>GMATVRLLDDAEISTLPEVKAVFDDIRATRGSDFVNNIWRGLANDPALLKRTWEQVKTVMVGEGALDPLTREMIYLAVSTANSCSYCAHSHTAAARAKGMTPAQHAEVLAIIGLAAQTNALV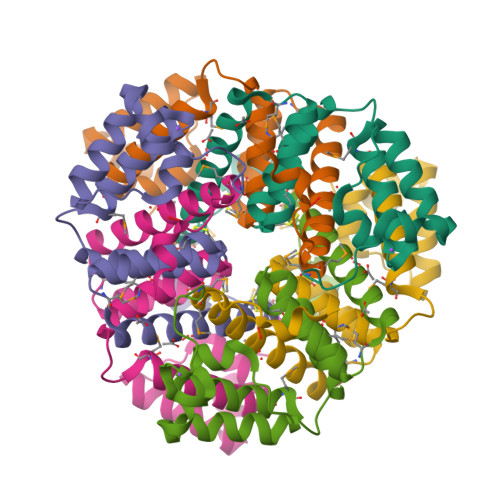TAMQIPVDEAFLVDGK[2x]> RS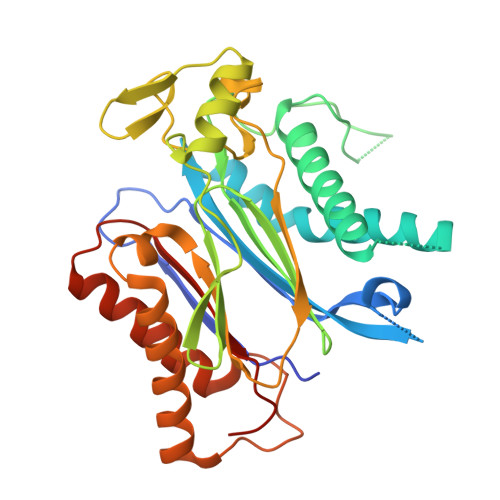VYELDCIPLWGTVSIQGNRSEMEDAFAVSPHFLKLPIKMLMGDHEGMSPSLTHLTGHFFGVYDGHGGHKVADYCRDRLHFALAEEIERIKDELCKRNTGEGRQVQWDKVFTSCFLTVDGEIEGKIGRAVVGSSDKVLEAVASETVGSTAVVALVCSSHIVVSNCGDSRAVLFRGKEAMPLSVDHKPDREDEYARIENAGGKVIQWQGARVFGVLAMSRSIGDRYLKPYVIPEPEVTFMPRSREDECLILASDGLWDVMNNQEVCEIARRRILMWHKKNGAPPLAERGKGIDPACQAAADYLSMLALQKGSKDNISIIVIDLKAQRKFKTRT>MAITAYSQQTRGLLGCIITSLTGRDKNQVEGEVQVVSTATQSFLATCVNGVCWTVYHGAGSKTLAGPKGPITQMYTNVDQDLVGWQAPPGARSLTPCTCGSSDLYLVTRHADVIPVRRRGDSRGSLLSPRPVSYLKGSSGGPLLCPSGHAVGIFRAAVCTRGVAKAVDFVPVESMETTMRMRKKKK[2x];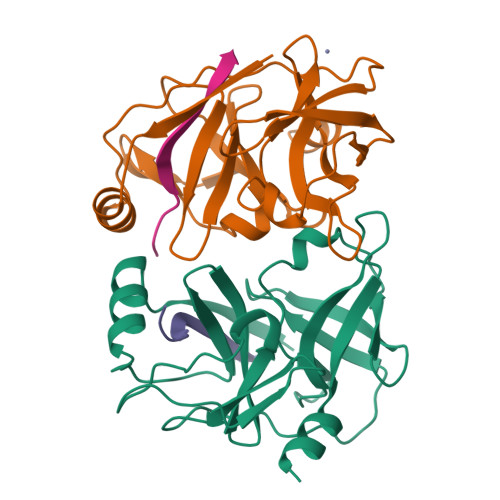>KGSVVIVGRIILSK[2x]>MKIKTLAIVVLSALSLSSTAALAAATTVNGGTVHFKGEVVNAACAVDAGSVDQTVQLGQVRTASLAQEG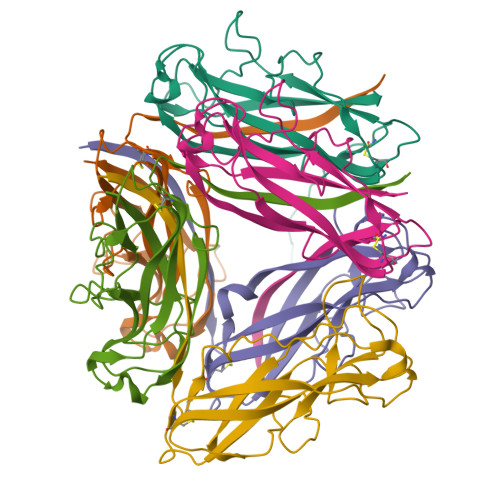ATSSAVGFNIQLNDCDTNVASKAAVAFLGTAIDAGHTNVLALQSSAAGSATNVGVQILDRTGAALTLDGATFSSETTLNNGTNTIPFQARYFATGAATPGAANADATFKVQYQ[6x]>MVYYPKKYELYKADEVPTEVVETDILIIGGGFSGCGAAYEAAYWAKLGGLKVTLVEKAAVERSGAVAQGLSAINTYIDLTGRSERQNTLEDYVRYVTLDMMGLAREDLVADYARHVDGTVHLFEKWGLPIWKTPDGKYVREGQWQIMIHGESYKPIIAEAAKMAVGEENIYERVFIFELLKDNNDPNAVAGAVGFSVREPKFYVFKAKAVILATGGATLLFRPRSTGEAAGRTWYAIFDTGSGYYMGLKAGAMLTQFEHRFIPFRFKDGYGPVGAWFLFFKCKAKNAYGEEYIKTRAAELEKYKPYGAAQPIPTPLRNHQVMLEIMDGNQPIYMHTEEALAELAGGDKKKLKHIYEEAFEDFLDMTVSQALLWACQNIDPQEQPSEAAPAEPYIMGSHSGEAGFWVCGPEDLMPEEYAKLFPLKYNRMTTVKGLFAIGDCAGANPHKFSSGSFTEGRIAAKAAVRFILEQKPNPEIDDAVVEELKKKAYAPMERFMQYKDLSTADDVNPEYILPWQGLVRLQKIMDEYAAGIATIYKTNEKMLQRALELLAFLKEDLEKLAARDLHELMRAWELVHRVWTAEAHVRHMLFRKETRWPGYYYRTDYPELNDEEWKCFVCSKYDAEKDEWTFEKVPYVQVIEWSF[2x];>MPSFVNPEKCDGCKALERTACEYICPNDLMTLDKEKMKAYNREPDMCWECYSCVKMCPQGAIDVRGYVDYSPLGGACVPMRGTSDIMWTVKYRNGK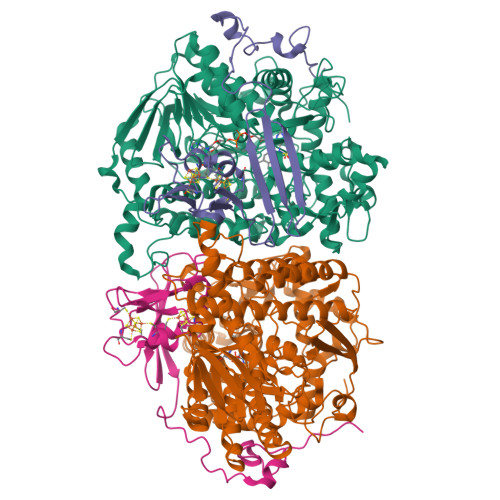VLRFKFAIRTTPWGSIQPFEGFPEPTEEALKSELLAGEPEIIGTSEFPQVKKKA[2x]> MRGSHHHHHHGSRIDYIEPFLDAASSVLRDMLLVENIEMGKPGLKSINQKIKGVSVIVGLAGSVEGSIIIDMDIETALFVASKLNFEEY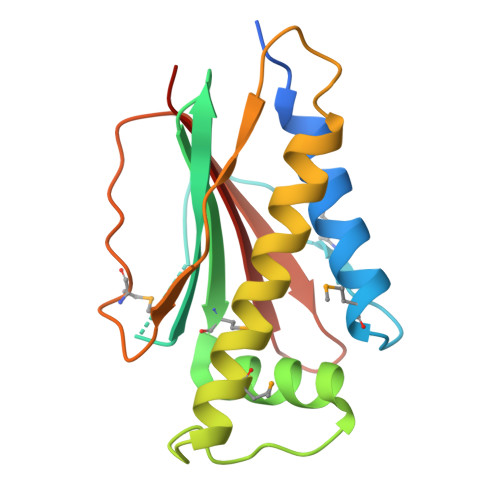DDFDDEETKEMVAATLTEVGNIIAGNFVTTLHAKGFVFDITPPAFIYGENMKISNKGSEALIVPFSLPDGKIIEVNIAIRERV>QFPRQCATVEALRSGMCCPDLSPVSGPGTDRCGSSSGRGRCEAVTADSRPHSPQYPHDGRDDREVWPLRFFNRTCHCNGNFSGHNCGTCRPGWRGAACDQRVLIVRRNLLDLSKEEKNHFVRALDMAKRTTHPLFVIATRRSEEILGPDGNTPQFENISIYNYFVWTHYYSVKKTFLGVGQESFGEVDFSHEGPAFLTWHRYHLLRLEKDMQEMLQEPSFSLPYWNFATGKNVCDICTDDLMGSRSNFDSTLISPNSVFSQWRVVCDSLEDYDTLGTLCNSTEDGPIRRNPAGNVARPMVQRLPEPQDVAQCLEVGLFDTPPFYSNSTNSFRNTVEGFSDPTGKYDPAVSSLHNLAHLFLNGTGGQVHLSPNDPIFVLLHTFTDAVFDEWLRRY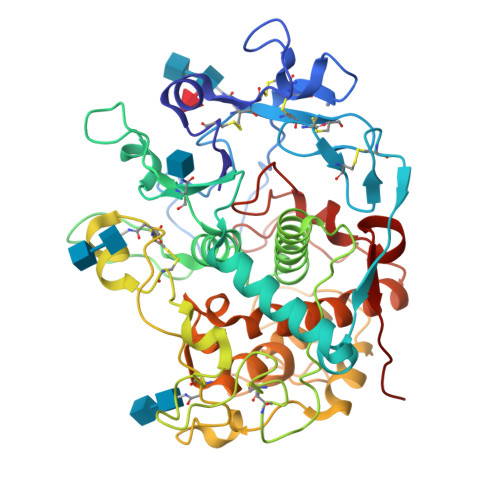NADISTFPLENAPIGHNRQYNMVPFWPPVTNTEMFVTAPDNLGYTYEIQWPS[4x]> GSEPEP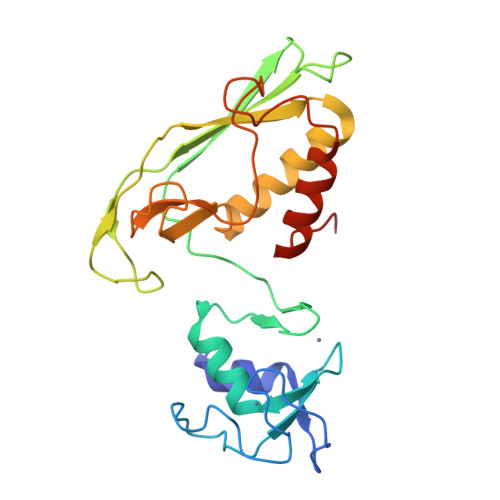EQVIKNYTEELKVPPDEDCIICMEKLSTASGYSDVTDSKAIGSLAVGHLTKCSHAFHLLCLLAMYCNGNKDGSLQCPSCKTIYGEKTGTQPQGKMEVLRFQMSLPGHEDCGTILIVYSIPHGIQGPEHPNPGKPFTARGFPRQCYLPDNAQGRKVLELLKVAWKRRLIFTVGTSSTTGETDTVVWNEIHHKTEMDRNITGHGYPDPNYLQNVLAELAAQGVTEDCLEQQ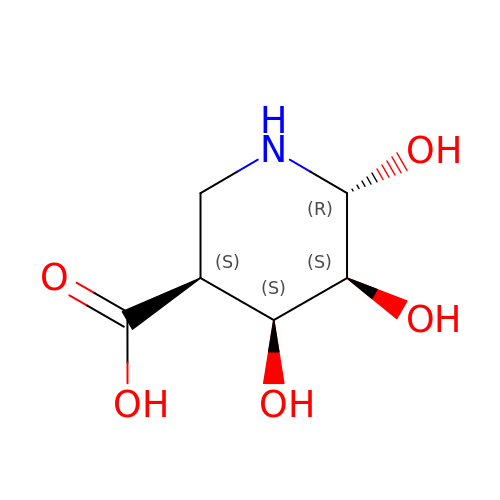(3~{S},4~{S},5~{S},6~{R})-4,5,6-tris(oxidanyl)piperidine-3-carboxylic acid | C6 H11 N O5 | ZIPHSWANMLXHEB-NEEWWZBLSA-N> MGRLLALVVGAALVSSACGGCVEVDSETEAVYGMTFKILCISCKRRSETNAETFTEWTFRQKGTEEFVKILRYENEVLQLEEDERFEGRVVWNGSRGTKDLQDLSIFITNVTYNHSGDYECHVYRLLFFENYEHNTSVVKKIHIEVVDKANRDMASIVSEIMMYVLIVVLTIWLVAEMIYCYKKIAAATETAAQENASEYLAITSESKENCTGVQVAE;> MHRDAWLPRPAFSLTGLSLFFSLVPPGRSMEVTVPATLNVLNGSDARLPCTFNSCYTVNHKQFSLNWTYQECNNCSEEMFLQFRMKIINLKLERFQDRVEFSGNPSKYDVSVMLRNVQPEDEGIYNCYIMNPPDRHRGHGKIHLQVLMEEPPERDSTVAVIVGASVGGFLAVVILVLMVVKCVRRKKEQKLSTDDLKTEEEGKTDGEGNPDDGAK;> MAQALLVPPGPESFRLFTRESLAAIEKRAAEEKAKKPKKEQDNDDENKPKPNSDLEAGKNLPFIYGDIPPEMVSEPLEDLDPYYINKKTFIVMNKGKAIFRFSATSALYILTPLNPVRKIAIKILVHSLFSMLIMCTILTNCVFMTLSNPPDWTKNVEYTFTGIYTFESLIKILARGFCLEDFTFLRDPWNWLDFSVIVMAYVTEFVSLGNVSALRTFRVLRALKTISVIPGLKTIVGALIQSVKKLSDVMILTVFCLSVFALIGLQLFMGNLRNKCLQWPPSDSAFETNTTSYFNGTMDSNGTFVNVTMSTFNWKDYIGDDSHFYVLDGQKDPLLCGNGSDAGQCPEGYICVKAGRNPNYGYTSFDTFSWAFLSLFRLMTQDYWENLYQLTLRAAGKTYMIFFVLVIFLGSFYLVNLILAVVAMAYEEQNQATLEEAEQKEAEFQQMLEQLKKQQEEAQAVAAASAASRDFSGIGGLGELLESSSEASKLSSKSAKEWRNRRKKRRQREHLEGNNKGERDSFPKSESEDSVKRSSFLFSMDGNRLTSDKKFCSPHQSLLSIRGSLFSPRRNSKTSIFSFRGRAKDVGSENDFADDEHSTFEDSESRRDSLFVPHRHGERRNSNVSQASMSSRMVPGLPANGKMHSTVDCNGVVSLVGGPSALTSPTGQLPPEGTTTETEVRKRRLSSYQISMEMLEDSSGRQRAVSIASILTNTMEELEESRQKCPPCWYRFANVFLIWDCCDAWLKVKHLVNLIVMDPFVDLAITICIVLNTLFMAMEHYPMTEQFSSVLTVGNLVFTGIFTAEMVLKIIAMDPYYYFQEGWNIFDGIIVSLSLMELGLSNVEGLSVLRSFRLLRVFKLAKSWPTLNMLIKIIGNSVGALGNLTLVLAIIVFIFAVVGMQLFGKSYKECVCKINDDCTLPRWHMNDFFHSFLIVFRVLCGEWIETMWDCMEVAGQTMCLIVFMLVMVIGNLVVLNLFLALLLSSFSSDNLAATDDDNEMNNLQIAVGRMQKGIDYVKNKMRECFQKAFFRKPKVIEIHEGNKIDSCMSNNTGIEISKELNYLRDGNGTTSGVGTGSSVEKYVIDENDYMSFINNPSLTVTVPIAVGESDFENLNTEEFSSESELEESKEKLNATSSSEGSTVDVVLPREGEQAETEPEEDLKPEACFTEGCIKKFPFCQVSTEEGKGKIWWNLRKTCYSIVEHNWFETFIVFMILLSSGALAFEDIYIEQRKTIKTMLEYADKVFTYIFILEMLLKWVAYGFQTYFTNAWCWLDFLIVDVSLVSLVANALGYSELGAIKSLRTLRALRPLRALSRFEGMRVVVNALVGAIPSIMNVLLVCLIFWLIFSIMGVNLFAGKFYHCVNMTTGNMFDISDVNNLSDCQALGKQARWKNVKVNFDNVGAGYLALLQVATFKGWMDIMYAAVDSRDVKLQPVYEENLYMYLYFVIFIIFGSFFTLNLFIGVIIDNFNQQKKKFGGQDIFMTEEQKKYYNAMKKLGSKKPQKPIPRPANKFQGMVFDFVTRQVFDISIMILICLNMVTMMVETDDQGKYMTLVLSRINLVFIVLFTGEFVLKLVSLRHYYFTIGWNIFDFVVVILSIVGMFLAEMIEKYFVSPTLFRVIRLARIGRILRLIKGAKGIRTLLFALMMSLPALFNIGLLLFLVMFIYAIFGMSNFAYVKKEAGIDDMFNFETFGNSMICLFQITTSAGWDGLLAPILNSAPPDCDPDTIHPGSSVKGDCGNPSVGIFFFVSYIIISFLVVVNMYIAVILENFSVATEESAEPLSEDDFEMFYEVWEKFDPDATQFIEFSKLSDFAAALDPPLLIAKPNKVQLIAMDLPMVSGDRIHCLDILFAFTKRVLGESGEMDALRIQMEDRFMASNPSKVSYEPITTTLKRKQEEVSAAIIQRNFRCYLLKQRLKNISSNYNKEAIKGRIDLPIKQDMIIDKLNG

Voltage-gated sodium (NaV) channels generate rapid sodium influx to initiate and propagate action potentials in excitable cells. NaV1.3 is involved in numerous physiological processes including neuronal development, hormone secretion and pain perception. NaVs are composed of a large pore-forming α-subunit and regulatory β-subunits. Here we report structures of human NaV1.3/β1/β2 in complex with clinically-used drug bulleyaconitine A and selective antagonist ICA121431.

To investigate how BLA modulates NaV1.3, we determined the 3.3 Å cryo-EM structure of NaV1.3/β1/β2 complexed with BLA. Strikingly, unambiguous density located in the central cavity of NaV1.3 close to the fenestration between DI and DII was observed, which fits well with BLA. BLA was sequestered in the cavity by extensive polar and non-polar interactions from P-loops and S6 helices from DI and DII. The binding was strengthened by five hydrogen bonds between BLA and carbonyl oxygens of T381, C941 and G942, and sidechains of Q382 and N972. The receptor site is defined by M380, T381, V416, I419 and L420 from DI, and C941, G942, M968, N972 and L976 from DII. No direct interaction from DIII or DIV was observed for BLA binding in our structure. The key residues F1759 and Y1766 are away from BLA at distances of 8.1 Å and 4.3 Å, respectively, which indicates that the receptor site for site-2 neurotoxins is distinct from that for local anesthetic and anti-arrhythmic drugs. The functionally closed activation gate of the complex structure shows that the gate is too small for BLA to access the central cavity. We therefore postulate that BLA binding stabilizes the open conformation of S6 of DI and DII at least, which may improve the open probability of the channel. Furthermore, the bulky BLA partially blocks the ion path, which would surely be an obstacle for conducting hydrated-Na+.> MQLRRYAATLSEGDIIVIPSSFPVALKAASDLNMVGIGVNAENNERNFLAGHKENVIR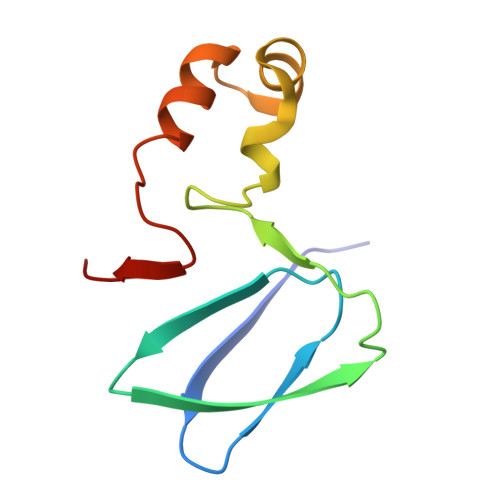QIPRQVSDLTFPGSGEEVEELLENQKESYFVDGQP>MASMTGGQQMGRIQADYEAKLAKYQADLAKYQKDLADYPVKLKAYEDEQTSIKAALAELEKHKNEDGNLTEPSAQNLVYDLEPNANLSLTTDGKFLKASAVDDAFSKSTSKAKYDQKILQLDDLDITNLEQSNDVASSMELYGNFGDKAGWSTTVSNNSQVKWGSVLLERGQSATATYTNLQNSYCNGKKISKIVYKYTVDPKSKFQGQKVWLGIFTDPTLGVFASAYTGQVEKNTSIFIKNEFTFYDEDGKPINFDNALLSVASLNREHNSIEMAKDYSGKFVKISGSSIGEKNGMIYATDTLNFKQGEGGSRWTMYKNSQAGSGWDSSDAPNSWYGAGAIKMSGPNNYVTVGATSATNVMPVSDM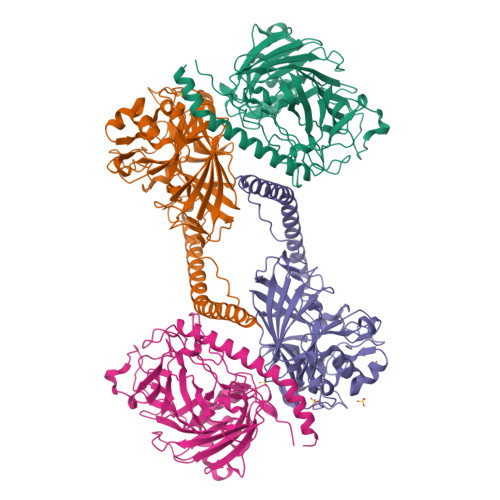PVVPGKDNTDGKKPNIWYSLNGKIRAVNVPKVTKEKPTPPVKPTAPTKPTLEHHHHHH[4x]> GAMGCVSSKSTTVLSPQTSFNEASRTSFRALPGPSQRQLEVYDQCLIGAARWPDDSSKSNTPENRAYCQSMYNSIRSAGDEISRGGITSFEELWGRATEWRLSKLQRGEPLYSAFASERTSDTDAVTPLVKPYKSVLARVVDHEDAHDEIMQDNLFGDLNVKVYRQTAYLHGNVIPLNTFRVATDTEYLRDRVAHLRTELGAKALKQHLQRYNPDRIDHTNASYLPIIKDHLNDLYRQAISSDLSQAELISLIARTHWWAASAMPDQRGSA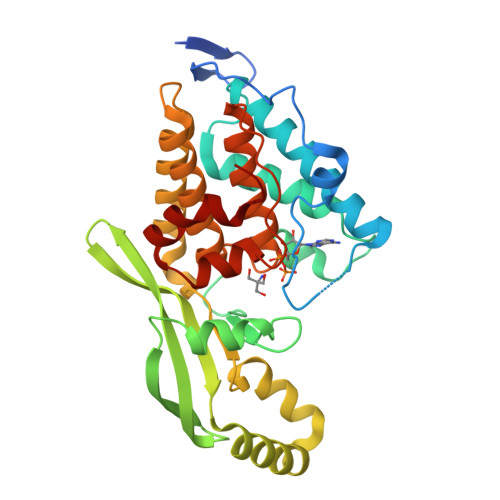AKAEFAARAIASAHGIELPPFRNGNVSDIEAMLSGEEEFVEKYRSLLDSDCF> GHMLSKRDAILKAAVEVFGK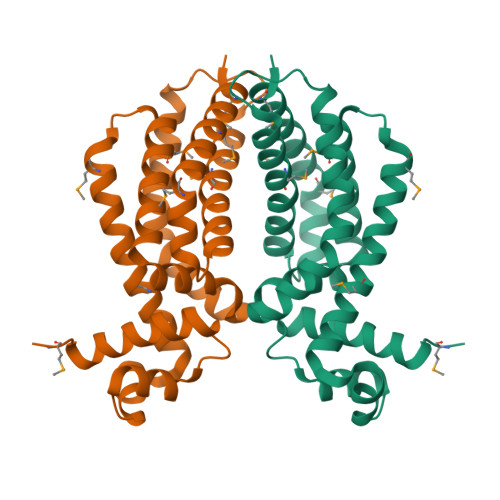KGYDRATTDEIAEKAGVAKGLIFHYFKNKEELYYQAYMSVTEKLQKEFENFLMKNRNRDIFDFMERWIEKKLEYSASHPEEADFLITLVSVDEGLRKRILLDLEKSQRVFFDFVREKLKDLDLAEDVTEEIALKFLMWFFSGFEEVYLRTYQGKPELLKRDMNTLVEEVKVMLRILKKGMTK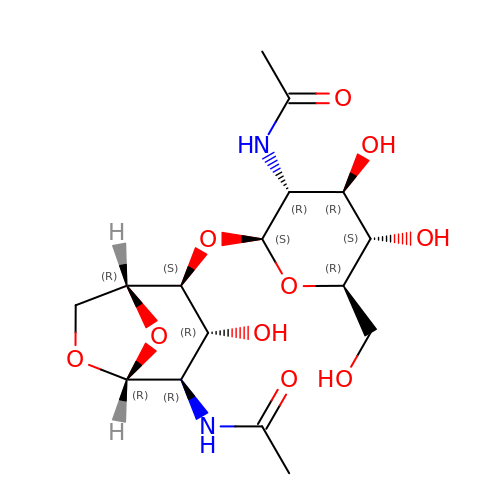N-[(1R,2S,3R,4R,5R)-2-[(2S,3R,4R,5S,6R)-3-acetamido-6-(hydroxymethyl)-4,5-bis(oxidanyl)oxan-2-yl]oxy-3-oxidanyl-6,8-dioxabicyclo[3.2.1]octan-4-yl]ethanamide | C16 H26 N2 O10 | UVQRTGABPMLDOA-KSKNGZLJSA-N>DVSGTVCLSALPPEATDTLNLIASDGPFPYSQDGVTFQNRESVLPTQSYGYYHEYTVITPGARTRGTRRIITGEATQEDYYTGDHYATF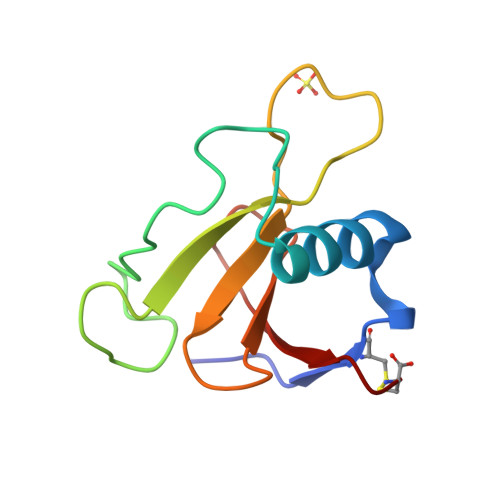SLIDQTC[2x]> VNMEYTKEKKVGEGTYAVVYLGCQHSTGRKIAIKEIKTSEFKDGLDMSAIREVKYLQEMQHPNVIELIDIFMAYDNLNLVLEFLPTDLEVVIKDKSILFTPADIKAWMLMTLRGVYHCHRNFILHRDLKPNNLLFSPDGQIKVADFGLARAIPAPHEILTSNVVTRWYRAPELLFGAKHYTSAIDIWSVGVIFAELMLRIPYLPGQNDVDQMEVTFRALGTPTDRDWPEVSSFM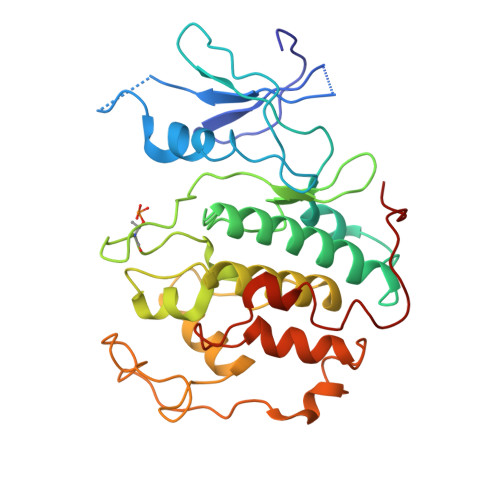TYNKLQIYPPPSRDELRKRFIAASEYALDFMCGMLTMNPQKRWTAVQCLESDYFKELPPPSDPSSIK MurAA catalyzes the first committed step of peptidoglycan synthesis, transferring an enolpyruvate moiety from phosphoenolpyruvate (PEP) to UDP-N-acetylglucosamine to produce UDP-GlcNAc-enolpyruvate and inorganic phosphate. MurAA comprises two domains with the active site Cys119 located in a flexible loop (Ala114–Ile126) that is solvent exposed in the ligand-free state. We refer to the domain containing the active site loop as the “catalytic domain” (residues 21–232) and the other as the “C-terminal domain” (residues 1–20, 233–419).

FOS inhibits MurAA by blocking access to the catalytic site making Cys119 inaccessible to PEP. Fosfomycin is an irreversible inhibitor of MurAA and is structurally analogous to the substrate PEP. Based on the structure of E. faecium MurAA, both the A149E and G220V mutations are located in the catalytic domain of the protein but distal from the active site. In addition to being quite distant from the active site, positions 149 and 220 are proximal to each other, and are both surface exposed, suggesting that these mutations could comprise part of a protein surface involved in interactions with other proteins. The structures of E. faecium MurAA with FOS–UDP-GlcNAc and by serendipity UDP–MurNAc suggest that, like other members of the MurA family, the protein transitions from an open to closed conformation upon UDP-GlcNAc binding.

>MEEIIVRGGNQLNGTVRIEGAKNAVLPILAASLLAEEGITTLDNVPILSDVFTMNQVIRHLNVDVDFDEQKNQVTIDASRQLEIEAPYEYVSQMRASIVVMGPLLARNGHAKVAMPGGCAIGKRPIDLHLKGFQALGAKIIQKNGYIEAIADELIGNTIYLDFPSVGATQNIMMAAVKAKGTTIIENVAREPEIVDLANILNKMGAQVYGAGTETMRIEGVDHLHAVNHSIVQDRIEAGTFMVAAAMTQGNVLIADAISEHNRPLISKLIEMGAEIIEEEGGVRVIGPKHILPTDVKTMPHPGFPTDMQAQMTAIQLVAEGTSVVTETVFENRFQHLEEMRRMNAHVKIDGNVAIMDGNHELQGAEVYATDLRAAAALVLAGLKANGITRVRNLNYLDRGYYNFHIKLQQLGADVERVDMDQTSAEKTAQTIA[4x]>MSLLPRTTSVKPGEKFDVIIVGLGPAAYGAALYSARYMLKTLVIGETPGGQLTEAGIVDDYLGLIEIQASDMIKVFNKHIEKYEVPVLLDIVEKIENRGDEFVVKTKRKGEFKADSVILGIGVKRRKLGVPGEQEFAGRGISYCSVADAPLFKNRVVAVIGGGDSALEGAEILSSYSTKVYLIHRRDTFKAQPIYVETVKKKPNVEFVLNSVVKEIKGDKVVKQVVVENLKTGEIKELNVNGVFIEIGFDPPTDFAKSNGIETDTNGYIKVDEWMRTSVPGVFAAGDCTSAWLGFRQVITAVAQG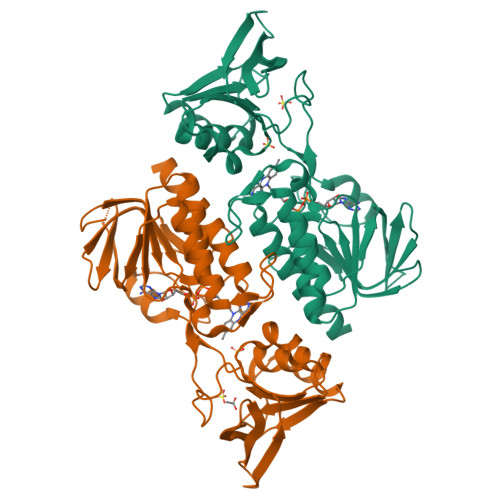AVAATSAYRYVTEKKGKK[4x]>GSHMAAEREETQQKVQDLETRNAELEHQLRAMERSLEEARAERERARAEVGRAAQLLDVS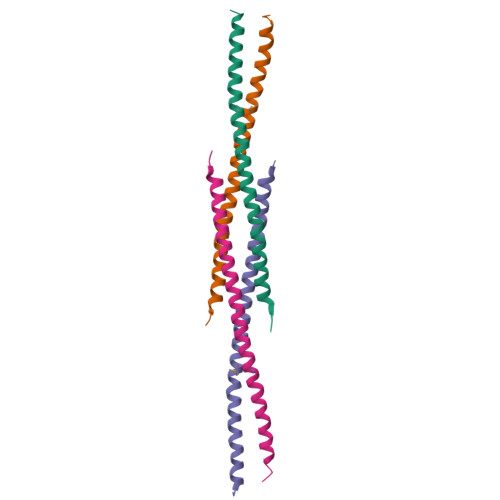LFELSELREGLARLAEAAP[4x]> MLTRNPIVPENHVSNPIVD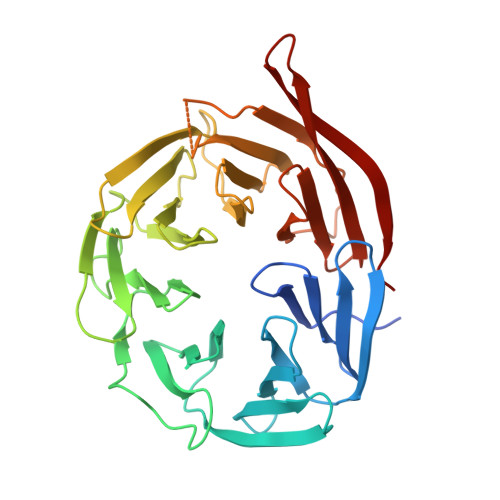YEFNQDQSCLIVSTPKSFDIYNVHPLKRIMSQEMPDAGTIRMLHRTNYIAFVSTKKELLHIWDDVKKQDITRVKLDAAVKDLFLSREFIVVSQGDVISIFKFGNPWNKITEDIKFGGVCEFANGLLVYSNEFNLGQIHVTRLQTDAEQVVGKGVLVKAHANPVKMVRLNRKGDMVATCSQDGTLIRVFQTDNGVLVREFRRGLDRTSIIDMRWSPDGSKLAVVSDKWTLHVFEVFNDGSGSGSGSGSEWSICNFKLKVSKGSNDCKIAWISDTGLVIVWPNRRLADTFKLNYNDDEHVWWLQLNQRNEIPL> MTTVKLTYFGHSAFHVEVDGVGIAIDPWITNPLSKTTLEDYLKNFKTDLVVITHAHEDHIGDALEIMRRTGAKFFSIHEIYVDLTQKGFQGIGANIGGPAKLDDVAPGLGIALTPATHSSYDKGVPTGAIIFKDGKALVYHAGDTGLFAEMQFIGELYAPKVALLPIGGHYTMDIEQALLATKLLRPEVVVPMHYNTFPPIRADPNEFKQKVESAGLAKVRVMEPGETVTFEFKGRQLGPEQKLISEEDLNSAVDHHHHHH

Igni18 is an enzyme of the hyperthermophilic Crenarchaeon Ignicoccus hospitalis, one of the most fascinating and enigmatic microorganisms known so far. While these enzymes apparently exert a rather specific function, Igni18, a promiscuous and primordial representative of the MβL family, could represent an example of a typical ancestral enzyme, because its structure and active site resemble the core of many modern specialized enzymes. The characterization of Igni18 conducted in this study unveiled high promiscuity and multi-functionality depending on the availability of different metal ions. Igni18 is highly promiscuous and thermostable and serves as a prototype to study the evolution of the remarkably diverse MβL superfamily.

Igni18 crystallized in space group R32 and crystals diffracted to 2.3 Å resolution. We solved the structure using a single SAD dataset. The overall fold of each monomer is composed of two mixed β-sheets (β14, β1, β2, β3, β4, β5, β6, and β7, β8, β9, β10, β11, β12, β13), slightly twisted and arranged in a parallel fashion in the center of the protein. Those are flanked by four helices on each side of the sheets (α1, α2, α3, α4 and α5, α6, α7, α8), thereby building the four-layered αββα core typical of the MβL superfamily. All interfaces between the three monomers have areas of ~850 Å2 with eleven intermolecular hydrogen bonds. Close beneath the protein surface and in direct vicinity to the loops connecting β4-α2, β10-α5, β11-α6, two Zn-ions are bound by His54, His56, His59, His118, His194, Asp58, and Asp144. The structure of Igni18 revealed two Zn2+ ions bound per monomeric unit. The inductively coupled plasma-mass spectrometry (ICP-MS) analysis conducted to verify the incorporated ion revealed that Zn is preferably bound to the recombinantly produced and purified, non-stripped protein Igni18 with 87.5% mass fraction (data available upon request). However, both methods did not result in binding poses in which cleavable bonds of the ligands approached the zinc ions closer than 7 Å. These results, alongside the fact that soaking the crystals with ligands remained unsuccessful, suggest that the loops surrounding the active center were not crystallized in a conformation receptive for ligand binding. The loop at the trimer interface (117–126, PVR5) exhibits the highest mobility in the monomer.> PKVDEDEEALK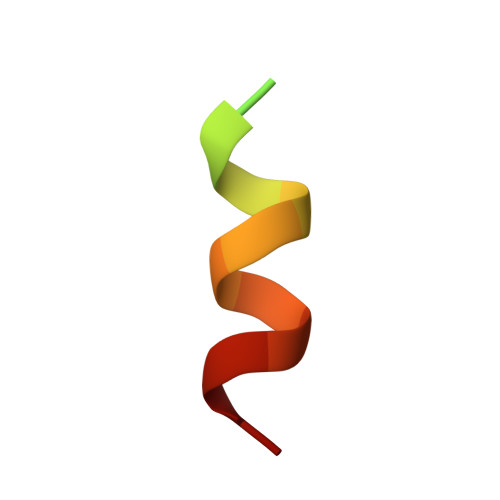QLAEWVS We recently characterized a novel roseophage, vB_DshS-R4C (R4C), that could infect the Dinoroseobacter shibae DFL12T, a ubiquitous group of Gram-negative α-proteobacteria of the Roseobacter clade. Here, we report the atomic capsid and in-situ structures of the tail machine of the marine siphophage, vB_DshS-R4C (R4C), which infects Roseobacter. The R4C virion, comprising 12 distinct structural protein components, has a unique five-fold vertex of the icosahedral capsid that allows genome delivery. In this study, we use cryo-electron microscopy (cryo-EM) and structure prediction to determine the atomic structure of the phage R4C capsid and the in-situ structure of the tail machinery to characterize the distinguished long rigid tail.

The adaptor docks to the stopper hexameric ring, with the latter formed by stopper proteins (vBDshSR4C_009) that maintain DNA inside the capsid. The stopper protein, a crucial module for head assembly, shares common structural features (anti-parallel β-strands barrel) with other siphophages, myophages and phage-like entities. The R4C stopper protein, with its long N-terminal extension, folds part of the N-terminus as an α-helix and plays a critical role in connecting the adaptor. Intriguingly, the R4C inter-stopper contact area (~274 Å2) formed by the N-termini, short loop, insertion loop and β2, seems too small for complex formation: we speculate that, similar to other tailed phages, the stopper proteins may exist as monomers in solution and form the stopper hexamer when incorporated into the head. After head assembly, the R4C stopper engages its long loop to fit inside a groove formed by the terminator, joining the head to the preassembled tail. As we described, the R4C terminator operates as a docking platform for the preassembled head and tail. Despite low sequence similarity, the R4C terminator protein shares a common structural topology with that of other long-tailed phages (e.g., λ phage gpU11, SPP1 gp1771), and integrates elements of a multi-stranded β-sheet barrel and two main helices at the periphery. The central α-helices and β3 cling to the neighbouring terminator surface, which is composed of an N-terminal helix, an insertion domain, and a segment of β1. The interaction between the R4C terminator and the tail tube relies chiefly on the tips of the terminator long β-hairpins binding to the minor groove, which is formed by adjacent tail tube subunits. Residue M50 in the β-hairpin tip inserts deeply into the hydrophobic cavity at the interaction interface to further stabilize layer coupling.

>MIESLADWSIFTDPDVFGEPVTWTTPPLPDPVPAIFTDASEDRPATLGPGVLTIAPTLTLGAAQLPFSPARNHRCTVRGITYRVAEVQPDGSGGLRLLLERV[6x];>[6x]MLKGKDGVVKNASTGDSIGHLQSWALDTQRDEVSGWGMGDDAERAFTTVGRASGNFEVYLDPADPSDDLEPGDLVDLELYPGGESTGSGYRSVAGALILSTAESASKDGIPMLTVNWRTSGALPQKATVS;>MSEAIIAAARGRLISPPFSDATGDVYRTPEAALPAIIVELDYTDAERISMGGGFIASAELRVEILAKRDDWSLLTPTPANTAEGMARLAALVRTAILAPPSDLSGLAWSIAPAGYEFETERGETPLARATQSFALQILQP[6x]>MLLAQKPFWQRHLAYPHINLDTVAHSLRLTGPLDTTLLLRALHLTVSEIDLFRARFSAQGELYWHPFSPPIDYQDLSIHLEAEPLAWRQIEQDLQRSSTLIDAPITSHQVYRLSHSEHLIYTRAHHIVLDGYGMMLFEQRLSQHYQSLLSGQTPTAAFKPYQSYLEEEAAYLTSHRYWQDKQFWQGYLREAPDLTLTSATYDPQLSHAVSLSYTLNSQLNHLLLKLANANQIGWPDALVALCALYLESAEPDAPWL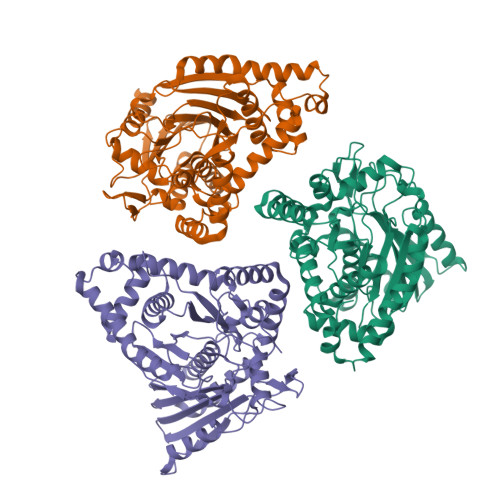WLPFMNRWGSVAANVPGLMVNSLPLLRLSAQQTSLGNYLKQSGQAIRSLYLHGRYRIEQIEQDQGLNAEQSYFMSPFINILPFESPHFADCQTELKVLASGSAEGINFTFRGSPQHELCLDITADLASYPQSHWQSHCERFPRFFEQLLARFQQVEQDVARLLAEPAALAATTSTRAIAS[3x]> GAGTAQEFVNCKIQPGKVVVFIKPTCPYCRRAQEILSQLPIKQGLLEFVDITATNHTNEIQDYLQQLTGARTVP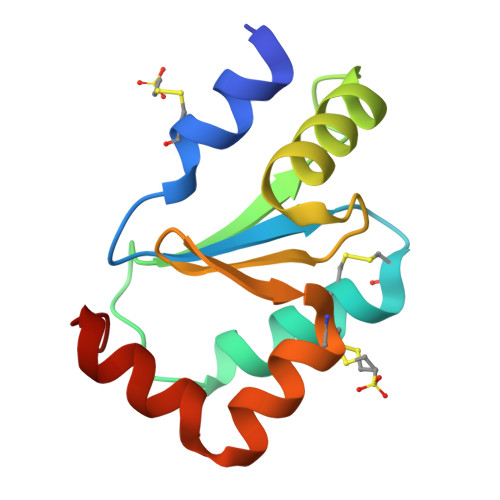RVFIGKDCIGGCSDLVSLQQSGELLTRLKQIGALQ> MRGSHHHHHHGS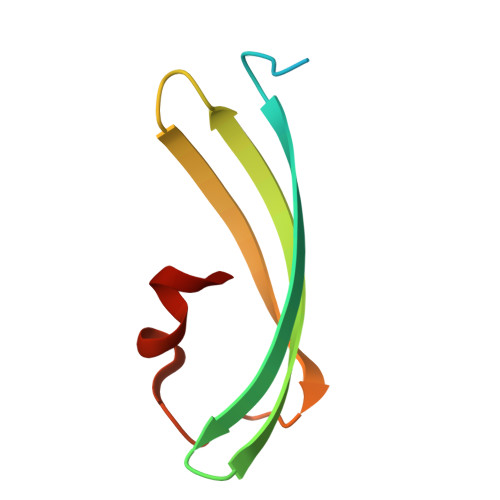ASFLKKTMPFKTTIEGTVNGHYFKCTGKGEGNPFEGTQEMKIEVIEGGPLPFAFHILSTSCX>[2x]PDCGVECKNETCTPKTVIYPDCGKNEKYEPPGDAKNTEINVINSGDKEGYIFEKLSEFCTNENNENGKNYEQWKCYYDNKKNNNKCKMEINIANSKLKNKVTSFDEFFDFWVRKLLIDTIKWETELTYCINNTDVTDCNKCNKNCVCFDKWVKQKEDEWTNIMKLFTNKHDIPKKYYLNINDLFDSFFFQVIYKFNEGEA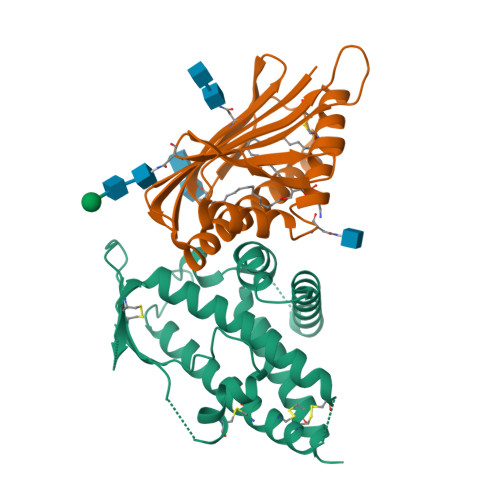KWNELKENLKKQIASSKANNGTKDSEAAIKVLFNHIKEIATICKDNNTNEG;>LQRLHMLQISYFRDPYHVWYQGNASLGGHLTHVLEGPDTNTTIIQLQPLQEPESWARTQSGLQSYLLQFHGLVRLVHQERTLAFPLTIRCFLGCELPPEGSRAHVFFEVAVNGSSFVSFRPERALWQADTQVTSGVVTFTLQQLNAYNRTRYELREFLEDTCVQYVQKHI[2x]(2S)-3-(1H-indol-3-yl)-N-[[1-(5-methoxypyridin-2-yl)cyclohexyl]methyl]-2-methyl-2-[(4-nitrophenyl)carbamoylamino]propanamide 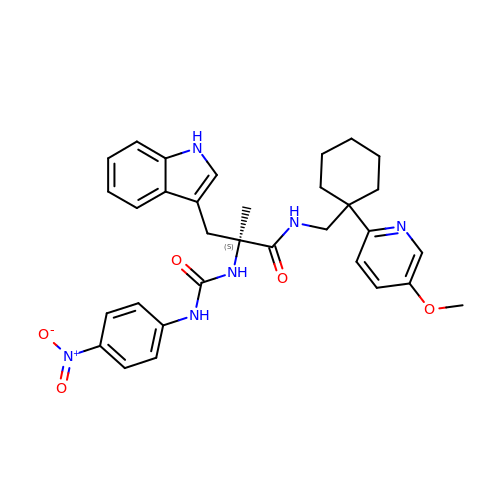| C32 H36 N6 O5 | NNFUWNLENRUDHR-HKBQPEDESA-N> MPASTYRLQISAEFTLFDAARIVPYLHRLGADWLYLSPLLESESGSSHGYDVVDHSRVDAARGGPEGLAELSRAAHERGMGVVVDIVPNHVGVATPKANRWWWDVLARGQRSEYADYFDIDWEFGGGRLRLPVLGDGPDELDALRVDGDE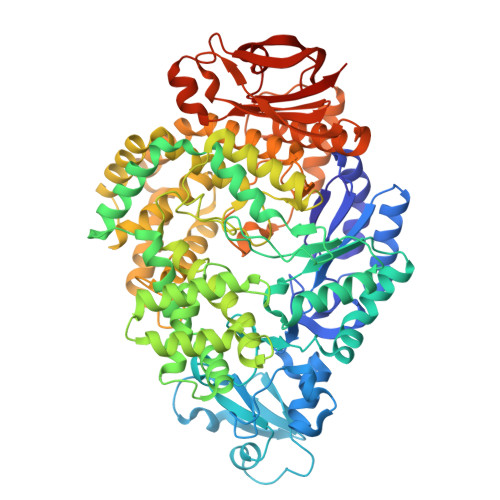LVYYEHRFPIAEGTGGGTPREVHDRQHYELMSWRRADHDLNYRRFFAVNTLAAVRVEDPRVFDDTHREIGRWIAEGLVDGLRVDHPDGLRAPGDYLRRLAELAQGRPIWVEKIIEGDERMPPQWPIAGTTGYDALAGIDRVLVDPAGEHPLTQIVDEAAGSPRRWAELVPERKRAVARGILNSEIRRVARELGEVAGDVEDALVEIAAALSVYRSYLPFGREHLDEAVAAAQAAAPQLEADLAAVGAALADPGNPAALRFQQTSGMIMAKGVEDNAFYRYPRLTSLTEVGGDPSLFAIDAAAFHAAQRDRAARLPESMTTLTTHDTKRSEDTRARITALAEAPERWRRFLTEVGGLIGTGDRVLENLIWQAIVGAWPASRERLEAYALKAAREAGESTDWIDGDPAFEERLTRLVTVAVEEPLVHELLERLVDELTAAGYSNGLAAKLLQLLAPGTPDVYQGTERWDRSLVDPDNRRPVDFAAASELLDRLDGGWRPPVDETGAVKTLVVSRALRLRRDRPELFTAYHPVTARGAQAEHLIGFDRGGAIALATRLPLGLAAAGGWGDTVVDVGERSLRDELTGREARGAARVAELFADYPVALLVETKLAAALEHHHHHH> AEYVRALFDHTGHDEQELPFKKGEILRIRDKPEEQLWNAENVEGKRGLIHVVLVEKYG

In this study, we incorporated a Cu2+-binding site into a natural protein domain, the 58 amino acid c-Crk-SH3, to create a miniaturized superoxide dismutase model, termed SO1. The miniprotein was found to be a strand-swapped dimer with an unusual coupled binuclear Type 2-like copper center in each protomer. SO1-Cu was found to be SOD-active with an activity only 1 order of magnitude lower than that of natural SOD enzymes and 1 to 2 orders of magnitude higher than that of other low-complexity SOD protein models of similar size. SOD proteins disproportionate superoxide into molecular oxygen and hydrogen peroxide and are part of the enzymatic machinery that protects the cell from oxidative stress.

The ‘different from design’ nature of SO1 required us to elucidate the structure of the engineered SH3 domain-derived protein. Using X-ray protein crystallography, we determined the three-dimensional structure of SO1 with bound Cu2+ by molecular replacement at 2.0 Å resolution (experimental details described in the SI and Table S1). The structure is well ordered and comprises all 58 SO1 residues. Surprisingly, the structure of SO1 does not show the anticipated compact SH3-like fold of the designed model. Instead, SO1 forms a homodimer in which strand β2 of the canonical SH3 fold and the adjacent loop regions are swapped with a symmetry-related molecule. In detail, part of the loop between strands β1 and β2 (RT Loop residues; hinge 1) starting at residues 15, strand β2 itself (residues 23–30) and the loop between β2 and β3 (n-Src Loop residues; hinge 2) up to residue 35 are involved in the strand swapping. Dimerization creates a new antiparallel β-sheet formed by residues 13 to 17 (strand β1b) and a short 310-helix before β3. Most interestingly, the dimeric structure shows two identical metal binding sites, each with two copper ions CuA and CuB. CuA is coordinated by NE2 of H10 and H13. CuB is located 3.6 Å apart from CuA and is coordinated by NE2 of H50 and the carboxyl group of E15. Additionally, CuA and CuB are coordinated by the E17′ carboxyl group, which is part of the symmetry-related protein chain forming the dimer.> GSMTSTVEFINRWQRIALLSQSLLELAQRGEWDLLLQQEVSYLQSIETVMEKQTPPGITRSI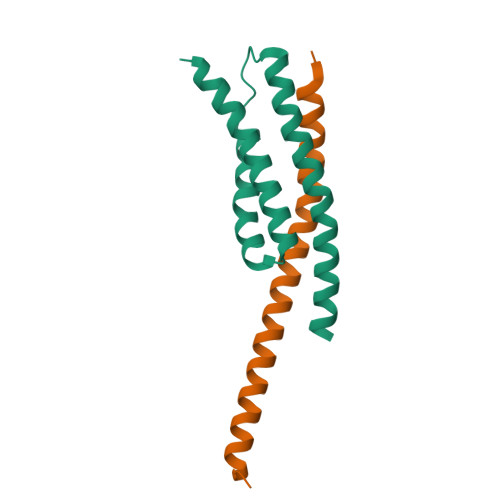QDMVAGYIKQTLDNEQLLKGLLQQRLDELSSLIG;> DGIIDNAQDNVNATLKSLTKQYLSVSNSIDETVARYKAQFTQLDTMMSKLNNTSSYLTQQFTAMNKS>[4x]M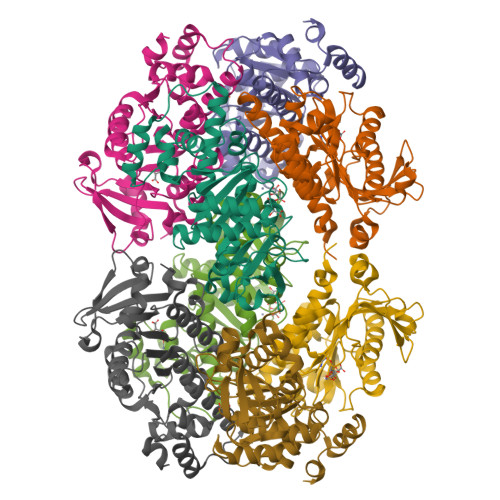QNITYSWFVQGMIKATTDAWLKGWDERNGGNLTLRLDDADIAPYHDNFHQQPRYIPLSQPMPLLANTPFIVTGSGKFFRNVQLDPAANLGIVKVDSDGAGYHILWGLTNEAVPTSELPAHFLSHCERIKATNGKDRVIMHCHATNLIALTYVLENDTAVFTRQLWEGSTECLVVFPDGVGILPWMVPGTDAIGQATAQEMQKHSLVLWPFHGVFGSGPTLDETFGLIDTAEKSAQVLVKVYSMGGMKQTISREELIALGKRFGVTPLASALAL> DGAVSSAT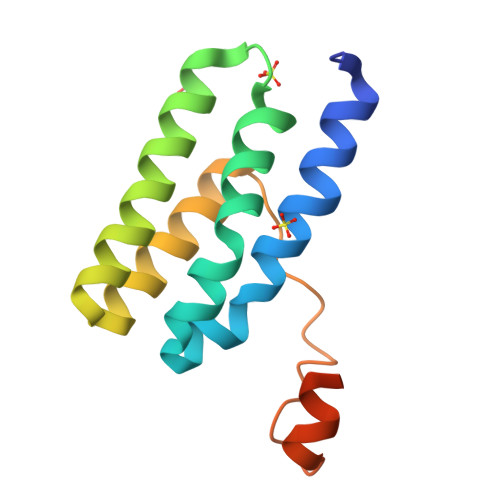INRARGLYGDRIAALKDAVAAGDFKAIAEEKNAFILFNSGAYPTNKAKKNAAIAQTNEIFKAIRSGDKAAVKSAYDAYMAANEIRPLPEINSNVGQGYSSEFDFRSRTKAGAIYVR>MKSLQALFGGTFDPVHYGHLKKVETLANLIGLTRVTIIPNNVPPHRPQPEANSVQRKHMLELAIADKPLFTLDERELKRNAPSVTAQTLKEWRQEQGPDVPLAFIIGQDSLLTFPTWDEYETILDNAHL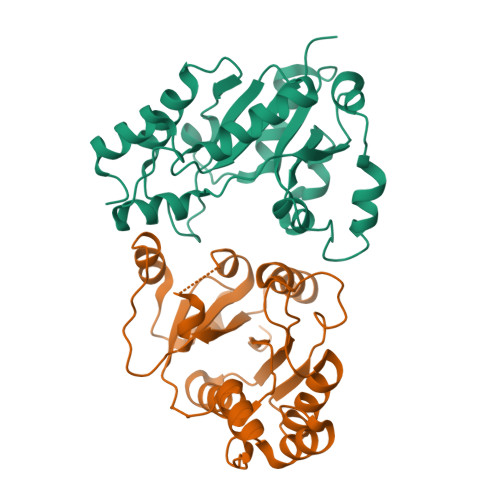IVLRRPGYPLEMAQPQYQQWLEDHLTHNPEDLHLQPAGKIYLAETPYFNISATIIRERLQNGESCEDLLPEPVLTYINQQGLYR[6x]>[2x]MAARGGRSEPPQLAEYSCSYTVSRPVYSELAFQQQRERRLPERRTLRDSLARSCSCSRKRAF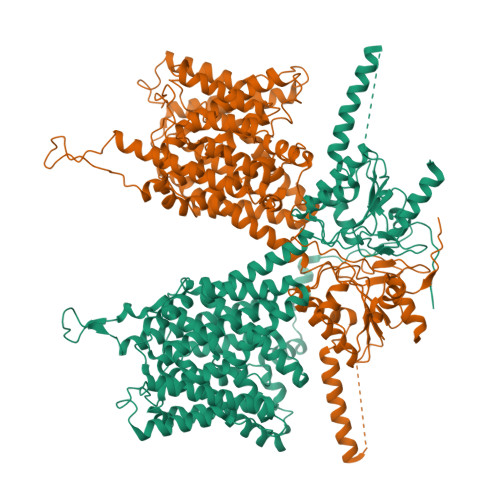GVVKTLLPILDWLPKYRVKEWLLSDIISGVSTGLVGTLQGMAYALLAAVPVQFGLYSAFFPILTYFVFGTSRHISVGPFPVVSLMVGSVVLSMAPDDHFLVPSGNGSALNSTTLDTGTRDAARVLLASTLTLLVGIIQLVFGGLQIGFIVRYLADPLVGGFTTAAAFQVLVSQLKIVLNVSTKNYNGILSIIYTLIEIFQNIGDTNIADFIAGLLTIIVCMAVKELNDRFKHRIPVPIPIEVIVTIIATAISYGANLEKNYNAGIVKSIPSGFLPPVLPSVGLFSDMLAASFSIAVVAYAIAVSVGKVYATKHDYVIDGNQEFIAFGISNVFSGFFSCFVATTALSRTAVQESTGGKTQVAGLISAVIVMVAIVALGRLLEPLQKSVLAAVVIANLKGMFMQVCDVPRLWKQNKTDAVIWVFTCIMSIILGLDLGLLAGLLFALLTVVLRVQFPSWNGLGSVPSTDIYKSITHYKNLEEPEGVKILRFSSPIFYGNVDGFKKCINSTVGFDAIRVYNKRLKALRRIQKLIKKGQLRATKNGIISDIGSSNNAFEPDEDVEEPEELNIPTKEIEIQVDWNSELPVKVNVPKVPIHSLVLDCGAVSFLDVVGVRSLRMIVKEFQRIDVNVYFALLQDDVLEKMEQCGFFDDNIRKDRFFLTVHDAILHLQNQVKSREGQDSLLETVARIRDCKDPLDLMEAEMNAEELDVQDEAMRRLAS>[2x]ATIEV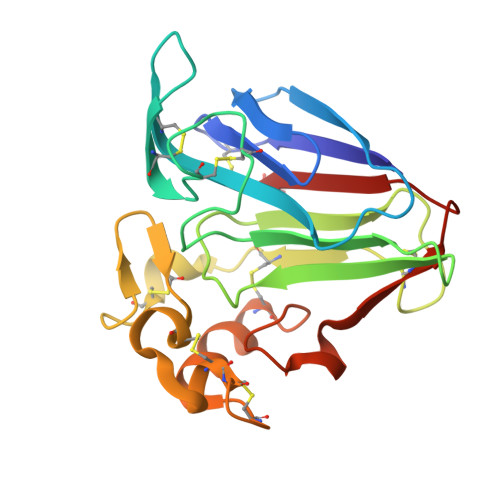RNNCPYTVWAASTPIGGGRRLDRGQTWVINAPRGTKMARVWGRTNCNFNAAGRGTCQTGDCGGVLQCTGWGKPPNTLAEYALDQFSGLDFWDISLVDGFNIPMTFAPTNPSGGKCHAIHCTANINGECPRELRVPGGCNNPCTTFGGQQYCCTQGPCGPTFFSKFFKQRCPDAYSYPQDDPTSTFTCPGGSTNYRVIFCP> GAEFMDLDQGGEALAPRQVLDLEDLVFTQGSHFMANKRCQLPDGSFRRQRKGYEEVHVPALKPKPFGSEEQLLPVEKLPKYAQAGFEGFKTLNRIQSKLYRAALETDENLLLCAPTGAGKTNVALMCMLREIGKHINMDGTINVDDFKIIYIAPMRSLVQEMVGSFGKRLATYGITVAELTGDHQLCKEEISATQIIVCTPEKWDIITRKGGERTYTQLVRLIILDEIHLLHDDRGPVLEALVARAIRNIECTQEDVRLIGLSATLPNYEDVATFLRVDPAKGLFYFDNSFRPVPLEQTYVGITEKKAIKRFQIMNEIVYEKIMEHAGKNQVLVFVHSRKETGKTARAIRDMCLEKDTLGLFLREGSASTEVLRTEAEQCKNLELKDLLPYGFAIHHAGMTRVDRTLVEDLFADKHIQVLVSTATLAWGVNLPAHTVIIKGTQVYSPEKGRWTELGALDILQMLGRAGRPQYDTKGEGILITSHGELQYYLSLLNQQLPIESQMVSKLPDMLNAEIVLGNVQNAKDAVNWLGYAYLYIRMLRSPTLYGISHDDLKGDPLLDQRRLDLVHTAALMLDKNNLVKYDKKTGNFQVTELGRIASHYYITNDTVQTYNQLLKPTLSEIELFRVFSLSSEFKNITVREEEKLELQKLLERVPIPVKESIEEPSAKINVLLQAFISQLKLEGFALMADMVYVTQSAGRLMRAIFEIVLNRGWAQLTDKTLNLCKMIDKRMWQSMCPLRQFRKLPEEVVKKIEKKNFPFERLYDLNHNEIGELIRMPKMGKTIHKYVHLFPKLELSVHLQPITRSTLKVELTITPDFQWDEKVHGSSEAFWILVEDVDSEVILHHEYFLLKAKYAQDEHLITFFVPVFEPLPPQYFIRVVSDRWLSCETQLPVSFRHLILPEKYPPPTELLDLQPLPVSALRNSAFESLYQDKFPFFNPIQTQVFNTVYNSDDNVFVGAPTGSGKTICAEFAILRMLLQSSEGRCVYITPMEALAEQVYMDWYEKFQDRLNKKVVLLTGETSTDLKLLGKGNIIISTPEKWDILSRRWKQRKNVQNINLFVVDEVHLIGGENGPVLEVICSRMRYISSQIERPIRIVALSSSLSNAKDVAHWLGCSATSTFNFHPNVRPVPLELHIQGFNISHTQTRLLSMAKPVYHAITKHSPK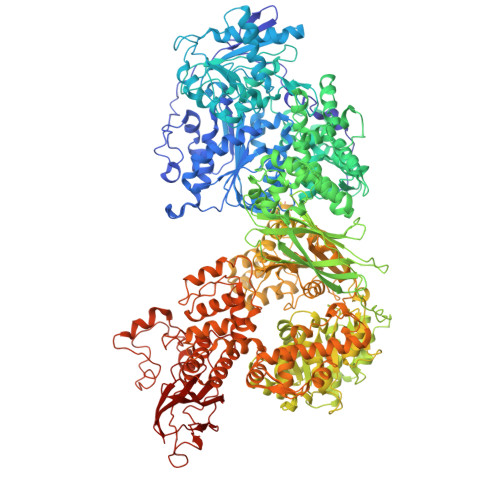KPVIVFVPSRKQTRLTAIDILTTCACDIQRQRFLHCTEKDLIPYLEKLSDSTLKETLLNGVGYLHEGLSPMERRLVEQLFSSGAIQVVVASRSLCWGMNVAAHLVIIMDTQYYNGKIHAYVDYPIYDVLQMVGHANRPLQDDEGRCVIMCQGSKKDFFKKFLYEPLPVESHLDHCMHDHFNAEIVTKTIENKQDAVDYLTWTFLYRRMTQNPNYYNLQGISHRHLSDHLSELVEQTLSDLEQSKCISIEDEMDVAPLNLGMIAAYYYINYTTIELFSMSLNAKTKVRGLIEIISNAAEYENIPIRHHEDNLLRQLAQKVPHKLNNPKFNDPHVKTNLLLQAHLSRMQLSAELQSDTEEILSKAIRLIQACVDVLSSNGWLSPALAAMELAQMVTQAMWSKDSYLKQLPHFTSEHIKRCTDKGVESVFDIMEMEDEERNALLQLTDSQIADVARFCNRYPNIELSYEVVDKDSIRSGGPVVVLVQLEREEEVTGPVIAPLFPQKREEGWWVVIGDAKSNSLISIKRLTLQQKAKVKLDFVAPATGAHNYTLYFMSDAYMGCDQEYKFSVDVKEAETDSDSD Rogdi is the human homolog of Drosophila melanogaster rogdi, and is a predicted leucine zipper protein of unknown function. The human Rogdi protein comprises 287 residues, and is highly conserved among species including fish, fly, frog, worm, and mouse. The crystal structure shows that Rogdi resembles a boomerang with an elongated curved structure comprising two distinct α and β domains. The α domain consists of four helices (H1 to H3, and H6) that form a left-handed four-helix bundle through van der Waals interactions.

However, we were unsuccessful in producing full-length selenomethionine (Se-Met) derivatized protein, due to poor protein expression in the methionine auxotrophic bacteria. Instead, Se-Met substituted Rogdi was produced and crystallized using N- and C-terminally truncated constructs (residues 11–276, referred to as tRogdi). The structure of tRogdi was determined by single-wavelength anomalous dispersion (SAD) and refined to 2.04 Å resolution. The structures of full-length and truncated Rogdi are almost identical, with a root mean square deviation (RMSD) of 0.8 Å for all Cα atoms. The N-terminal amino acids 48–55, which correspond to the direct linker between H1 and S1 in all molecules including tRogdi, RogdiH, and RogdiL, were not visible in the electron density map, indicating high flexibility.

> SGERAVLEEEFRWLLHDEVHAVLKQLQDILKEASLRFTLPGSGTEGPAKQENFILGSCGTDQVKGVLTLQGDALSQADVNLKMPRNNQLLHFAFREDKQWKLQQIQDARNHVSQAIYLLTSRDQSYQFKTGAEVLKLMDAVMLQLTRARNRLTTPATLTLPEIAASGLTRMFAPALPSDLLVNVYINLNKLCLTVYQLHALQPNSTKNFRPAGGAVLHSPGAMFEWGSQRLEVSHVHKVECVIPWLNDALVYFTVSLQLCQQLKDKIS> MRLVLEEPFKRLWNGRDPFEAVEALQGKVYRELEGRRTLRTEVDGRGYFVKIHRGIGWGEIAKNLLTA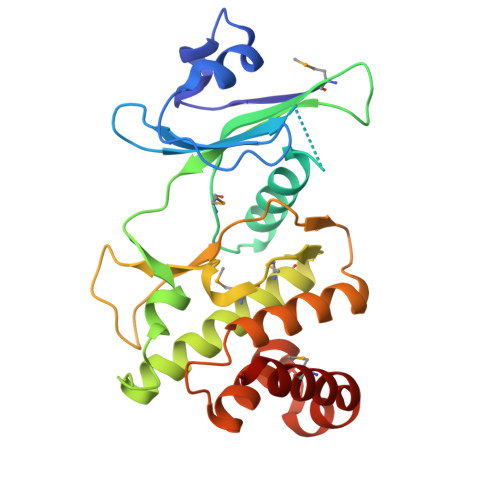KLPVLGARQEWQAIRRLHEAGVATMTAVAYGERGSDPARQHSFIVTEELAPTVDLEVFSQDWRERPPPPRLKRALVEAVARMVGDMHRAGVNHRDCYICHFLLHTDKPVSADDFRLSVIDLHRAQTRDATPKRWRNKDLAALYFSALDIGLTRRDKLRFLRTYFRRPLREILRDEAGLLAWMERKAEKLYE> MTEFDEIVKPDDKEETSESTEENLESTEETSESTEESTEESTEESTEDKTVETIEEENEN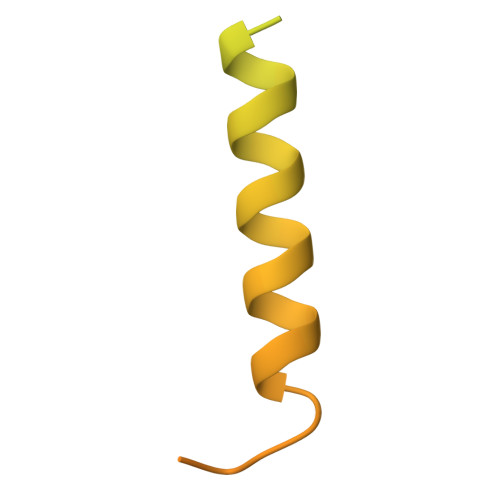KLEPTTTDEDSSKFDPVVLEQRIASLEQQVTTFLSSQMQQPQQVQQTQSDVTESNKEDNDYSDEELVDKLDLD> GAMGSGEPQSPSRRVFNPYTEFKEFSRKQIKDMEKMFKQYDAGRDGFIDLMELKLMMEKLGAPQTHLGLKNMIKEVDEDFDSKLSFREFLLIFRKAAAGELQEDSGLCVLARLSEIDVSS

EFhd1 and EFhd2 are homologous EF-hand proteins with similar structures. Although separately localized within cells, both are actin-binding proteins that modulate F-actin rearrangement through Ca2+-independent actin-binding and Ca2+-dependent actin-bundling activity. EFhd1Zn, EFhd2Zn and EFhd1Ca comprised two EF-hands, a ligand mimic (LM) helix at the C-terminus, a PR region at the N-terminus and a C-terminal linker. In addition, we determined that EFhd1 and EFhd2 bind actin independently of Ca2+ or Zn2+ and also exhibit Ca2+-dependent and Zn2+-dependent actin-bundling activity.

To obtain EFhd2Zn, we added EGTA and EDTA to final molar concentrations 15 times higher (0.18 mM each) than that of the protein to the EFhd2 proteins to remove native ions and then dialyzed the proteins. Thereafter, ZnCl2 was added to the protein solution to a final concentration of 0.75 mM. At a wavelength near the Zn K-edge (λ = 1.2851 Å/9648 eV), the Ca2+ f″ and Zn2+ f″ were 0.9 and 0.5 electrons, respectively. For that reason, we cannot rule out the possibility that the anomalous signals for EFhd2Zn originated from Ca2+, because the wavelength for the EFhd2Zn data collection was near the Zn K-edge [Fig. 1(g)]. We used a single EFhd2Zn crystal to collect datasets at the peak and remote positions of the Zn K-edge, which are termed EFhd2Zn(P) or EFhd2Zn(R), respectively. After calculation of the anomalous difference maps for each dataset, the anomalous difference map for EFhd2Zn(R) was subtracted from that for EFhd2Zn(P) to calculate the ΔAno map. The peak heights of the ΔAno map calculated from EFhd2Zn(P) and EFhd2Zn(R) were 11.1 and 9.3σ in EF1 and EF2, respectively [Figs. 1(h) and 1(i)]. In addition, we confirmed that Zn2+ mediates crystal-packing interactions between EFhd2 molecules, which raises the possibility of the involvement of Zn2+-mediated multimerization in AD.>[2x]VSSCSEDWVGYQRKCYFISTVKRSWTSAQNACSEHGATLAVIDSEKDM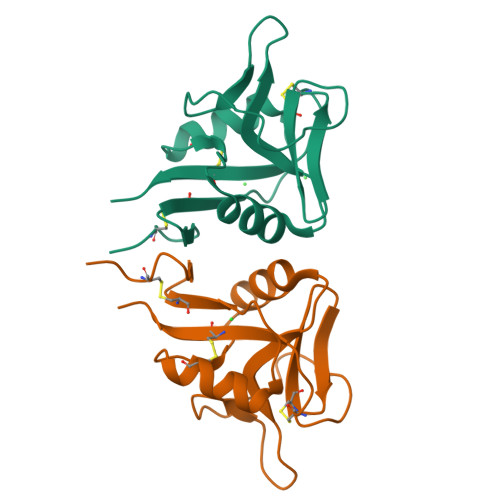NFLKRYAGREEHWVGLKKEPGHPWKWSNGKEFNNWFNVTGSDKCVFLKNTEVSSMECEKNLYWICNKPYK> MSGIALSRLAQERKAWRKDHPFGFVAVP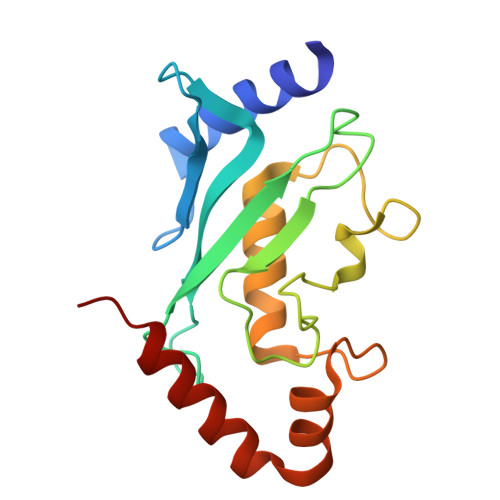TKNPDGTMNLMNWECAIPGKKGTPWEGGLFKLRMLFKDDYPSSPPKCKFEPPLFHPNVYPSGTVSLSILEEDKDWRPAITIKQILLGIQELLNEPNIQDPAQAEAYTIYCQNRVEYEKRVRAQAKKFAPS> ADTRIGVTIYKYDDNFMSVVRKAIEKDGKSAPDVQLLMNDSQNDQSKQNDQIDVLLAKGVKALAINLVDPAAAGTVIEKARGQNVPVVFFNKEPSRKALDSYDKAYYVGTDSKESGVIQGDLIAKHWQANQGWDLNKDGKIQYVLLKGEPGHPDAEARTTYVVKELNDKGIQTEQLALDTAMWDTAQ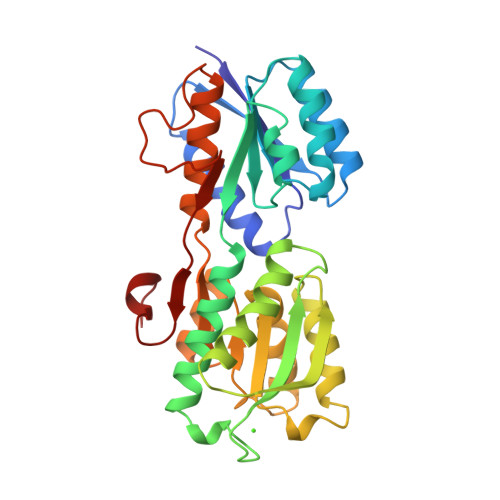AKDKMDAWLSGPNANKIEVVIANNDAMAMGAVEALKAHNKSSIPVFGVDALPEALALVKSGAMAGTVLNDANNQAKATFDLAKNLAEGKGAADGTSWKIENKIVRVPYVGVDKDNLSEFTQK>GPEPDMISVFIGTWNMGSVPPPKNVTSWFTSKGLGKTLDEVTVTIPHDIYVFGTQENSVGDREWLDLLRGGLKELTDLDYRPIAMQSLWNIKVAVLVKPEHENRISHVSTSSVKTGIANTLGNKGAVGVSFMFNGTSFGFVNCHLTSGNEKTARRNQNYLDILRLLSLGDRQLNAFDISLRFTHLFWFGDLNYRLDMDIQEILNYISRKEFEPLLRVDQLNLEREKHKVFLRFSEEEISFPPTYRYERGSRDTYAWHKQKPTGVRTNVPSWCDRILWKSYPETHIICNSYGCTDDIVTSDHSPVFGTFEVGV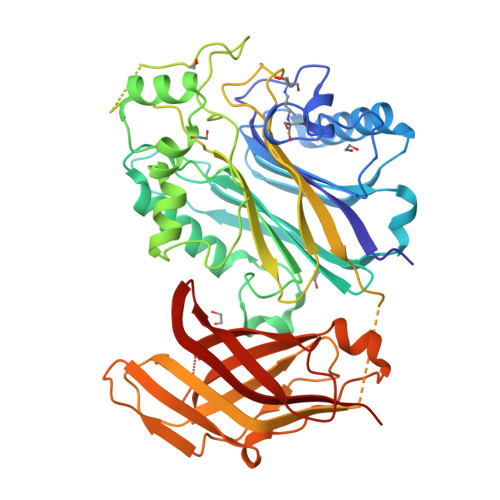TSQFISKKGLSKTSDQAYIEFESIEAIVKTASRTKFFIEFYSTCLEEYKKSFENDAQSSDNINFLKVQWSSRQLPTLKPILADIEYLQDQHLLLTVKSMDGYESYGECVVALKSMIGSTAQQFLTFLSHRGEETGNIRGSMKVRVPTER[8x]>VRRGDFVRNWQLVAAVPLFQKLGPAVLVEIVRALRARTVPAGAVICRIGEPGDRMFFVVEGSVSVATPNPVELGPGAFFGEMALISGEPRSATVSAATT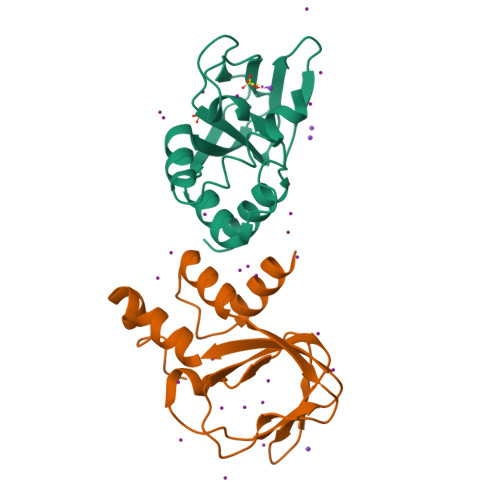VSLLSLHSADFQMLCSSSPEIAEIFRKTALEARGAAASA[2x]TRIETHYLAMMONIUM 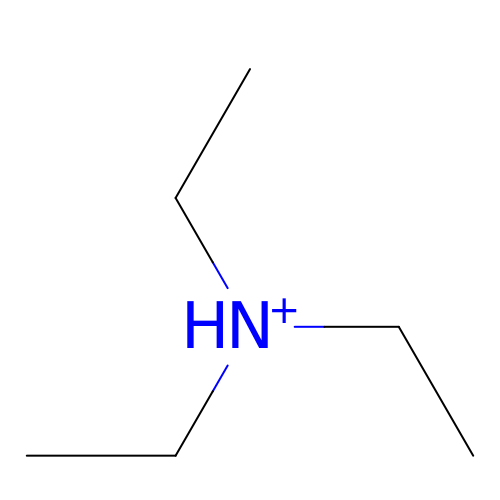ION | C6 H16 N | ZMANZCXQSJIPKH-UHFFFAOYSA-O> GSNNVLPTWSLDSNGEMRSRLSLSEVLDSGDLMKFAVDKTGCQFLEKAVKGSLTSYQKFQLFEQVIGRKDDFLKLSTNIFGNYLVQSVIGISLATNDDGYTKRQEKLKNFISSQMTDMCLDKFACRVIQSSLQNMDLSLACKLVQALPRDARLIAICVDQNANHVIQKVVAVIPLKNWEFIVDFVATPEHLRQICSDKYGCRVVQTIIEKLTADSMNVDLTSAAQNLRERALQRLMTSVTNRCQELATNEYANYIIQHIVSNDDLAVYRECIIEKCLMRNLLSLSQEKFASHVVEKAF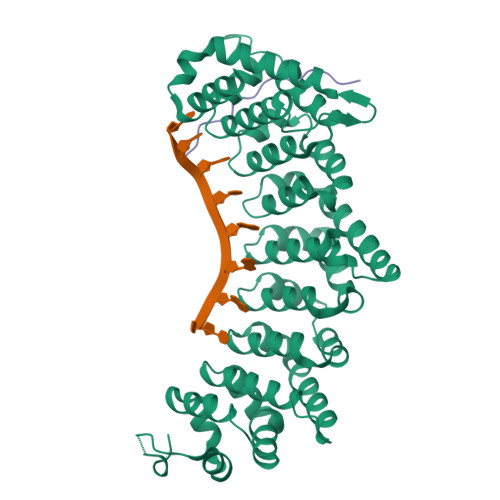LHAPLELLAEMMDEIFDGYIPHPDTGKDALDIMMFHQFGNYVVQCMLTICCDAVSGRRQTKEGGYDHAISFQDWLKKLHSRVTKERHRLSRFSSGKKMIETLANLRSTHPIYELQ;> GSNSSTIAYSKSQHEAPKQLLQLRSEIKPLIPLNQP>[2x]RNLLVQEGEEGFEVRSWPGTDGKSKTILLDNPEDAAQQKSIERFILANFDNFEQMPDELFLVDNKVLSHHDGRTRILARKEDGAWTYNANVELMSVTELLDAAHVSGKVRGESYQQVIDALTEYHASTAEHADYELTSVEKLLNLRKQVEGYVLGHPDSGRVQAMNALLNQVNSRLEAVSVLVVSEQSIKAHDSFSHLYDQLDNANLKESKHLYLDGNGDF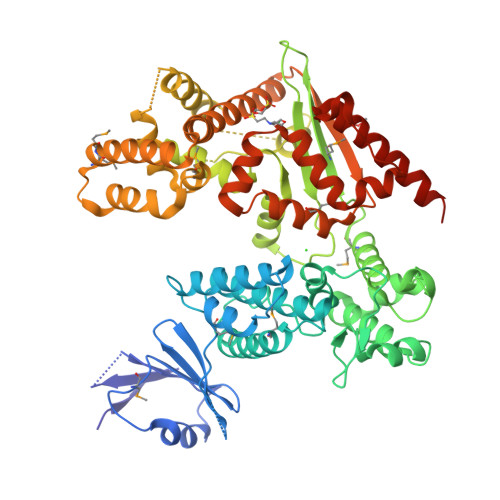VTKGKGNLANIDKLGGSDAVLEKVKAAVSHEYGQVVADTIFAGLSANDLAKDGKGIDIAGLNKVHQAIEQHMSPVSATMYIWKPSDHSALGHAALQIGQGRTQLEGQAAADFNKQNYVSWWPLGSKSSNIRNIFNVATEDQPDLKLRWSDFSQPAHQNDTLEHDMASEENDGFGLNDGETKLKRFVEKLNAAKGIDASYKDASEGYASVLLGNPDMLASTGIPAHVFQPFVDQWNDTSYDMMDVANRFAEELQKQAQASGDPALVEKRIDNVVRLFAERALEEIEAFKASQADEGRVFRINLEGLDVAAMQAEWNRLSNDPDARYQLLTKNASSTVAKVLKAGGADKLIGHTWRPKFGVWTPTELFNFGQALQEAQLEIAAKKQSHQATDLLDAL>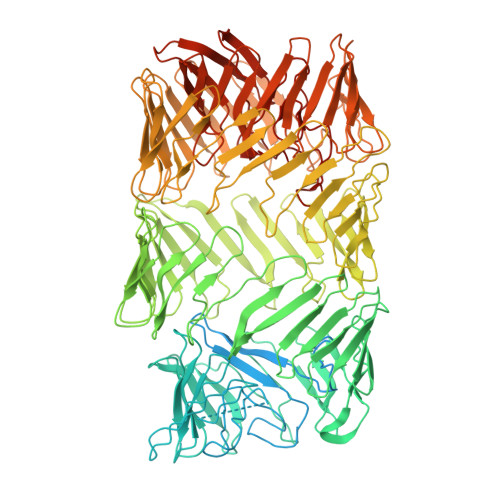 MGSSHHHHHHSQDPENLYFQSMIPQFVIPLTNCLGQSYHFSSQPIPKGEHKKFDSEQSAKAFLDDFVPLRSSRVEELYHLLGQFPPNVPDEELTPELYAPVFAKALVNGSLYVASFPKTKKNATISSEPTPVPKQVKAKSKQNKAHTSSKTQAKNSASAKPLQTGSECHEKAGDPVSLVTGEEILTLNDVELPNGFVWSRTYRSSKASRNQGLGYGWRHAFQFELKEVTDEKHNVTSWEFISDSADEIEFEPVEHGSTSYQVYVGASCHFLNPNIRIVTLSSGDQYRFELVEDIWLLKQVRNGIFSTFQLRYSRNHRLIEVAHNKRPVLECQYDKQGRLVELLNAKTEQVLTTYIYDEQDDLVGATNDLGLTERYEYQDQHLIAKRVRPTGFTHYFEWSGEGSSAKCIRNFGDSGIYDYRFHYEGAKSSYSDSLDNEWTFIHDEQGHLLEKSSPTGRTWQWHYDHLGRKEKAVFPDNSTTQYQYNQQGQLISKLHSSGAQIQYGYDSLGKLVKTVSPDGDLEKAYYNSLGQRVWDIDALGCVTEYEYDKHGQVVKRESEDGKKSRWWWDKQQRLVAHEVDGTLLRYSYGATDLVNGIAYPDGCVAQISYDDYGRRTSIRYFNDEDKVGYSEEYAYDEFSRVAQIQTPEGVTSYQWGALAQQEAVIFPDGSHISYEYDQQRNLTKLVRSDGLAFEFWYDSEGLLSGTVGFDGLHSQFKYDSMGRIIRKDVADRTVLYSYDDAGFLQHIKAGNGKNIVENHFNYTLGGRLTLASNRHQTLQYQYSSFGHLTKRIQGQFEIGEEFNRVGQRVSQTLPDKTSFNFSYDTNGRLSEIRFSDDSLPKIEFQYDVMGRLSVTETESFRESKLYDGVGRLVEQQWSGREKKYIYNAQNRISSILDNTAGATHYQYDTLGYVTKVSEAGSTSTFESDSFGNPALADSKVMSDRIEAYAGVRYKYDQQGNQVKREGDGTVQKRVFDALSQLVEVHGDSSISHYEYDALGRRTKKITQNGITEFLWEGERLLGERTADGFRWYLYQPETYIPLAVLENGSIYLYECDQVGKPERLKDSAGNIVWSASYDVHGFASIDVEEVRNPLRFQGQYFDQETNLHYNLARYYDPKLGRFIQQDPISIAGGINHYQYAVNPIQWIDPTGF> GEIQWMRPSKEVGYPIINAPSKTKLEPSAFHYVFEGVKEPAVLTKNDPRLKTDFEEAIFSKYVGNKITEVDEYMKEAVDHYAGQLMSLDINTEQMCLEDAMYGTDGLEALDLSTSAGYPYVAMGKKKRDILNKQTRDTKEMQKLLDTYGINLPLVTYVK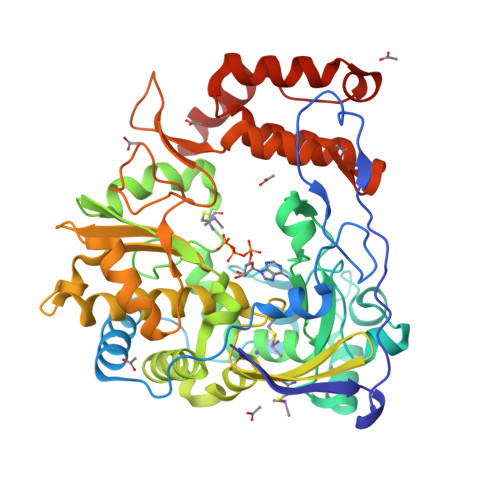DELRSKTKVEQGKSRLIEASSLNDSVAMRMAFGNLYAAFHKNPGVITGSAVGCDPDLFWSKIPVLMEEKLFAFDYTGYDASLSPAWFEALKMVLEKIGFGDRVDYIDYLNHSHHLYKNKTYCVKGGMPSGCSGTSIFNSMINNLIIRTLLLKTYKGIDLDHLKMIAYGDDVIASYPHEVDASLLAQSGKDYGLTMTPADKSATFETVTWENVTFLKRFFRADEKYPFLIHPVMPMKEIHESIRWTKDPRNTQDHVRSLCLLAWHNGEEEYNKFLAKIRSVPIGRALDLPEYSTLYDRWLDSF>[3x]MRKVLGVLAGLVLGIPGVAAE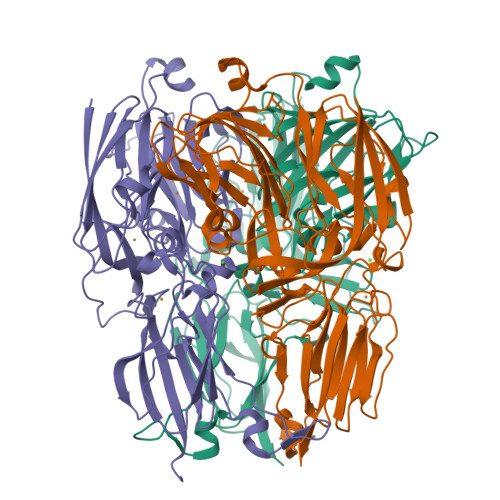RHFTLEARSSIFEVDQGVYLRGFSFNDMSPGPMLVVEEGDTVHITLRNLDNVTHGLSIHAANTQTSRFLGNVQPGETREFSFTADFPGVFMYHCAPGGHGIMAHTMGGQFGMIVVEPKEKYRMERELGRGPDLKLYIIQSEAYASGRDFYDGKALYVMFNGRNFRYVDEPIPVRPGDYLRIYFLNVGPNLTSTLHVVGGIFEYMYYQGNPKNLVVGAQTALAGPSDSWVIEWRVPPVEGDYTLVTHVFGTAIKGALGILRAKKDAPRIPEVRAEGVPGVKEIPASAKRVVDPYGLASPGHEHTVRVPLDPALAQPVAVGAKALEPLPVTVQMVGNSFYPKVLEIPVGTTVEFVNEDVFDLLEGERTGRHDAVVIDVQGPEPFVTPKLGHGERYRITFTKPGEYVYICSIHPYMKGIIRVYEPLSQRADSQ>[6x]MGSDKIHHHHHHMASSKQADPQTD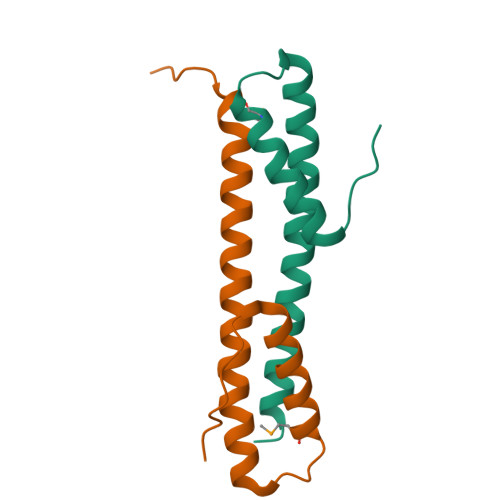ARPLPQDFETALAELESLVSAMENGTLPLEQSLSAYRRGVELARVCQDRLAQAEQQVKVLEGDLLRPLDPAALDDE>DDQLKQSALDFHEFPVPGKIQVSPTKPLATQRDLALAYSPGVAAPCLEIEKDPLKAYKYTARGNLVAVISNGTAVLGLGNIGALAGKPVMEGKGVLFKKFAGIDVFDIEVDELDPDKFIEVVAALEPTFGGINLEDIKAPECFYIEQKLRERMNIPVFHDDQHGTAIISTAAILNGLRVVEKNISDVRMVVSGAGAAAIACMNLLVALGLQKHNIVVCDSKGVIYQGREPNMAETKAAYAVVDDGKRTLDDVIEGADIFLGCSGPKVLTQEMVKKMARAPMILALANPEPEILPPLAKEVRPDAIICTGRSDYPNQVNNVLCFPFIFRGALDVGATAINEEMKLAAVRAIAELAHAEQSEVVASAYGDQDLSFGPEYIIPKPFDPRLIVKIAPAVAKAAMESGVATRPIADFDVYIDKLTEFVYKTNLFMKPIFSQARK[2x]

While reducing NAD(P)+ to NAD(P)H, MEs catalyze the oxidative decarboxylation of the TCA cycle intermediate L-malate to produce the TCA carbon source pyruvate and a byproduct carbon dioxide (CO2) in the presence of divalent metal ions such as a magnesium (Mg2+) ion. The hybrid-type MEs consist of an N-terminal catalytic domain (ME domain) and a C-terminal activity regulating domain. The PTA domain does not possess an enzymatic activity of PTA but acts as an allosteric modulator of catalysis; that is, binding of some metabolites to the PTA domain increases or decreases the enzymatic activity. Binding of acetyl-CoA to the PTA domain is known to reduce the catalytic activity of several hybrid-type MEs.

To obtain a more physiologically relevant state structure, we added the cofactors NADP+ and MgCl2 to EcMaeBapo solution prior to data collection and determined its structure (EcMaeBholo) at 2.73 Å resolution. While the cryo-EM map of EcMaeBholo clearly shows the PTA domain, the map around the ME domain is unclear. Furthermore, in 2D classification of EcMaeBholo data, the ME domain was ambiguous. These results of the cryo-EM map and 2D classification indicate the flexibility of the ME domain of EcMaeB. Consequently, the catalytic site of EcMaeBholo including cofactors could not be modeled well although we added NADP+ and Mg2+ to the sample. Therefore, we had to conduct further local refinement of the ME domain dimer to observe cryo-EM maps of NADP+ and the Mg ion.>[4x]QSVEESEGGLFKPTDTLTLTCTASGFSLSGHGVIWVRQAPGKGLE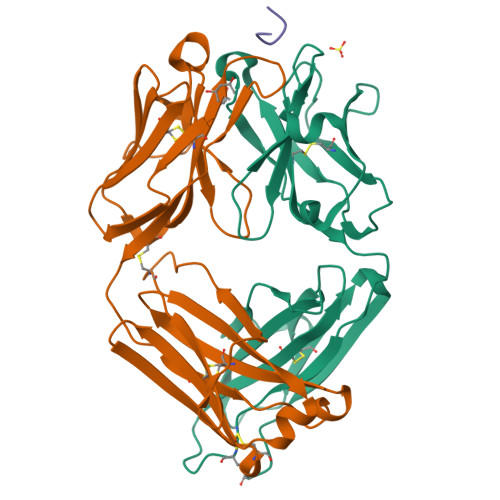WIGSAGAYGRIYYASWAKSRSTITRNTNLNTVTLKMTSLTAADTATYFCARRSDVGTSVGFDSWGPGTLVTISSSSGQPKAPSVFPLAPCCGDTPSSTVTLGCLVKGYLPEPVTVTWNSGTLTNGVRTFPSVRQSSGLYSLSSVVSVTSSSQPVTCNVAHPATNTKVDKTVAPSTCSHHHHHH;>[4x]DMTQTPSSKSVPVGDTVTINCQASESVYSNNRLSWFQQKPGQPPKLLIYLVSTLASGVPSRFKGSGSGTQFTLTISDVVCDDAATYYCVGYKSSTTDGLAFGGGTEVVVKGDPVAPTVLIFPPAADQVATGTVTIVCVANKYFPDVTVTWEVDGTTQTTGIENSKTPQNSADCTYNLSSTLTLTSTQYNSHKEYTCKVTQGTTSVVQSFNRGDC;>RNIIXGSDS[4x]>MVQPWAWQVASLADRYEESFDIGAAVEPHQLNGRQGKVLKHHYNSIVAENAMKPISLQPEEGVFTWDGADAIVEFARKNNMNLRFHTLVWHNQVPDWFFLDEEGNPMVEETNEAKRQANKELLLERLETHIKTVVERYKDDVTAWDVVNEVVDDGTPNERGLRESVWYQITGDEYIRVAFETARKYAGEDAKLFINDYNTEVTPKRDHLYNLVQDLLADGVPIDGVGHQAHIQIDWPTIDEIRTSMEMFAGLGLDNQVTELDVSLYGWPPRPAFPTYDAIPQ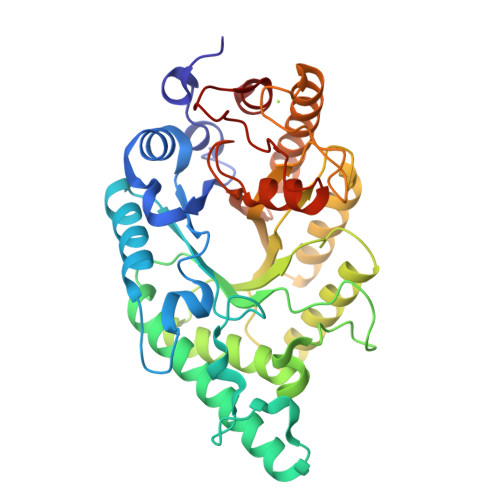ERFQAQADRYNQLFELYEELDADLSSVTFWGIADNHTWLDDRAREYNDGVGKDAPFVFDPNYRVKPAFWRIID[2x]>[15x]SFPEVVELNVGGQVYFTRHSTLISIPHSLLWKMFSPKRDTANDLA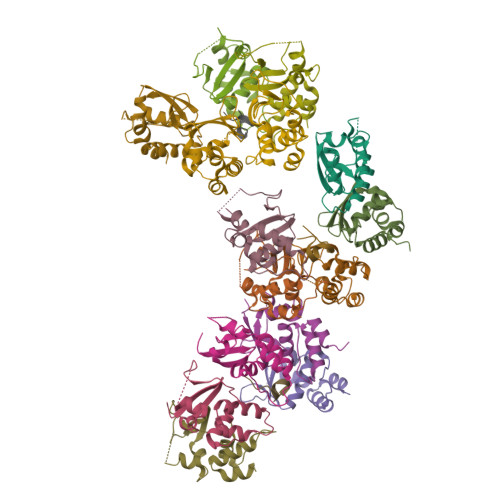KDSKGRFFIDRDGFLFRYILDYLRDRQVVLPDHFPEKGRLKREAEYFQLPDLVKLLTPDEIKQSPDEF;>QLPILHHAYLPSIGG[3x]> AHHHHHHMQGSVTEFLKPRLVDIEQVSSTHAKVTLEPLERGFGHTLGNALRRILLSSMPGCAVTEVEIDGVLHEYSTKEGVQEDILEILLNLKGLAVRVQGKDEVILTLNKSGIGPVTAADITHDGDVEIVKPQHVICHLTDENASISMRIKVQRGRGYVPASTRIHSEEDERPIGRLLVDACYSPVERIAYNVEAARVEQ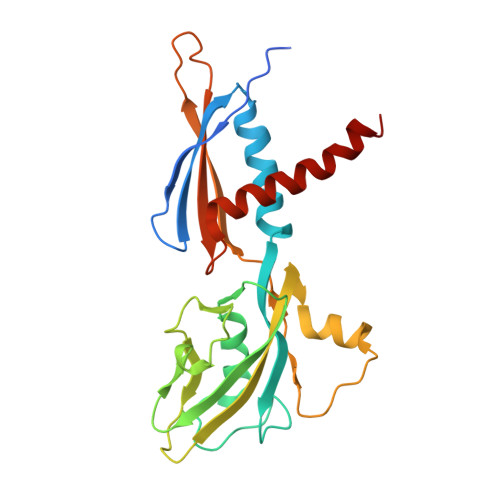RTDLDKLVIEMETNGTIDPEEAIRRAATILAEQLEAFVDLR>[8x]GPLGSDHSLNIVTVTLNMERHHFLGISIVGQSNDRGDGGIYIGSIMKGGAVAA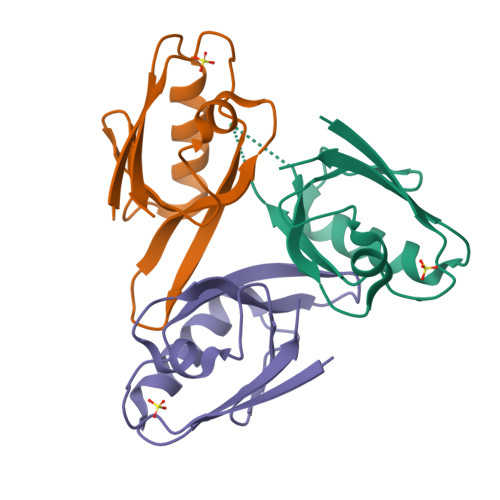DGRIEPGDMLLQVNDVNFENMSNDDAVRVLREIVSQTGPISLTVAKATD>MAKEKARYFTFLLYPESIPSDWELKLETLGVPMAISPLHDKDKSSIKGQKYKKAHYHVLYIAKNPVTADSVRKKIKLLLGEKSLAMVQVVLNVENMYLYLTHESKDAIAKKKHVYDKADIKLINNFDIDRYVTLDVEEKTELFNVVVSLIRAYTLQNIFDLYDFIDENGETYGLTINLVNEVIAGKTGFMKLLFDGAYQRSKRGTKNEER[3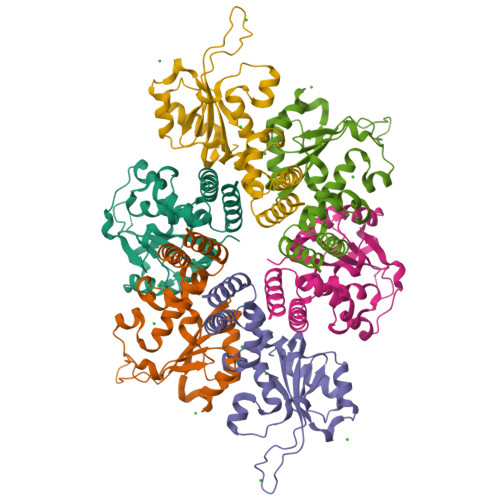x]> MGSSHHHHHHSSGENLYFQGHMEAIQTHPANAAQAKAFTAPGSLSFPGGASEIANSTAPTNGASNGG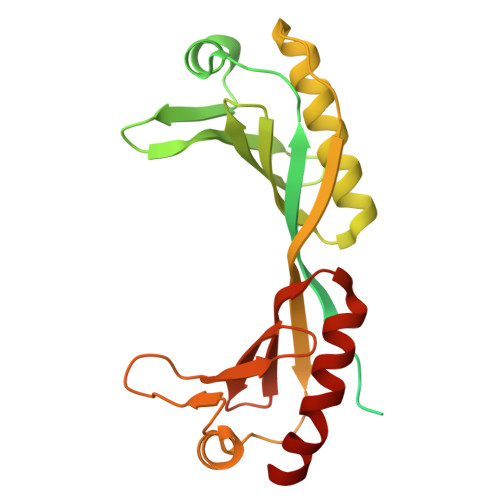QQQGVQATSGAGVTPATPAATPGAGPAGPSGITPTLQNIVATVNLDCRLDLKTIALHARNAEYNPKRFAAVIMRIREPKTTALIFASGKMVVTGAKSEDDSKLASRKYARIIQKLGFNAKFTDFKIQNIVGSCDIKFPIRLEGLASKHHNFSSYEPELFPGLIYRMIKPKIVLLIFVSGKIVLTGAKVREEIYQAFEMIYPVLQDFRKV>[2x]MAHHHHHHMSQADIEPIVYLSVASREELVPLSEARVPVLDRGFIFGDGVYEVVPIYAEGARRAPFRIAQHLARLARSLKKIGIADPHDEAGWRALVARLVDANAAALGDGQHAIVYIQVTRGVAKRG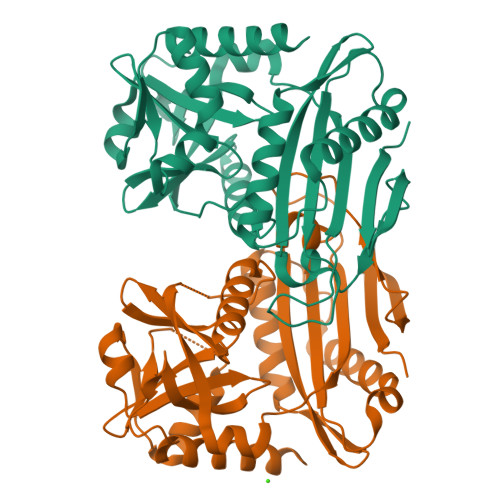HAFPANAVPTVFAMASPLALPTDAQRAQGVHCVTAEDRRWLHCDIKSVSLLGNVLMAQHAAEHDAAETIQLRDGNVTEGSSSNVWIVKNGELIAPPRSNRILEGIRYALVEELAEECGIRFVAREINEAELRAADEILLTSATKEILPVTRLDDLPVQGGRPGPVFDALYAAYQRAKAHEMESV> MVKIYLIEHVIGAVAYDENGNIVDYITNPRDLGKITEELLNNEKGIPFSATVELLKKVNPQEVVVENEAEVPKLQALGYRVSYEPYSKVSRIFRESLPKVAIDIKFASNEEDYYNFLHELSLEYTRRKLRSAAQKRDLLAIQAVRAMDDIDKTINLFSERLREWYSIHFPELDKLIEDHEEYATIVSRFGDRGFLTIDSLKELGFNEQRINRILDAAKKSIGADISEDDLSAMRMIANTILDLYNIRRNLNNYLEGVMKEVAHHH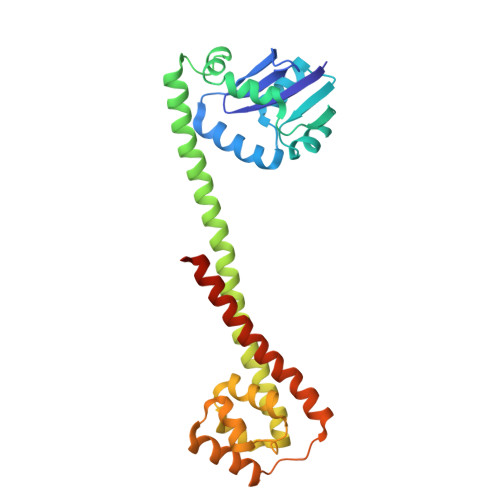HHH>[4x]APIKVGINGFGRIGRMVFQAICDQGLIGTEIDVVAVVDMSTNAEYFAYQMKHDTVHGRPKYTVEAVKSSPSVETADV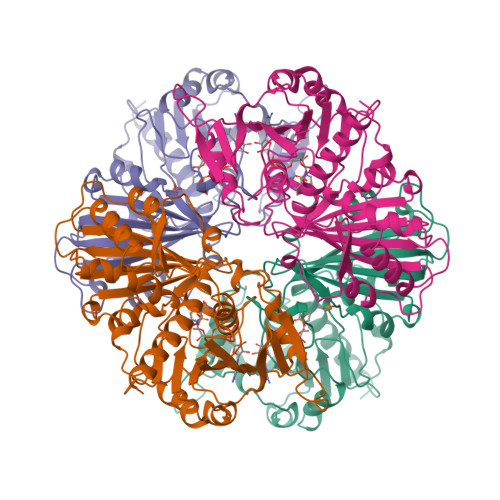LVVNGHRIKCVKAQRNPADLPWGKLGVDYVIESTGLFTDKLKAEGHIKGGAKKVVISAPASGGAKTIVMGVNQHEYSPASHHVVSNASCTTNCLAPIVHVLTKENFGIETGLMTTIHSYTATQKTVDGVSLKDWRGGRAAAVNIIPSTTGAAKAVGMVIPSTKGKLTGMSFRVPTPDVSVVDLTFRATRDTSIQEIDKAIKKAAQTYMKGILGFTDEELVSADFINDNRSSVYDSKATLQNNLPGEKRFFKVVSWYDNEWAYSHRVVDLVRYMAAKDAASS> MSHFFADHDAPLSMLSVKTEYFPQLTDKEQKYAHFMSKASHAGSRVVMRQVSHE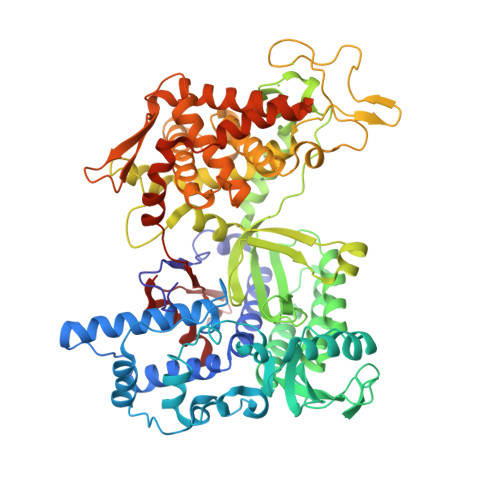SEPIFDLILAIHSKLNGKYPEDDITQKQQTGLYLEYVSQFLSNLGNFKSFGDTKFIPRCEVKFFKQLLELAKINPSSSPLTLSPVDVNHEFTSHHLFSTINELIDIGIYHVEEKAALLGFPSQGYTSAYYLGLPVTPEDMALLKEQLFAELAILPENTRINKVGENSFQIWVASENVKNQITETYPSGQITLSNAVTKVEFIFGDHSREMRLVASYLKEAQKFAANDTQKAMLQEYINHFVTGSSQAHKEAQKLWVKDISPVIETNIGFIETYREPSGIIGEFESLVAIQNKERTAKFSSLVNNAEEFISLLPWSKDYEKPIFNPPDFTSLEVLTFTGSGIPAGINIPNYDDVRLKIGFKNVSLGNILSAAAKSSSKHPPSFISQEDRPIFEKYQSDSFEVQVDIHELLGHGSGKLLTEFTDGFNFDKENPPLGLDGKPVSTYYKVGETWGSKFGQLAGPFEECRAEVIAMFLLTNKKILDIFGFHDVESQDKVIYAGYLQMARAGLLALEYWNPKTGKWGQPHMQARFSIMKTFMKHSTDKNFLKLEMNSTNDDFAIKLDKSLIKTAGHECVKDYLKHLHVYKCSGDVEQGSKYFIDRSTVTPDLASLRDIVLSKRLPRRQFIQSNSYIDDNNKVTLKEYDETPQGMLQSFLDREL>[4x]HPNYKLTYFNMRGRAEIIRYIFAYLDIQYEDHRIEQA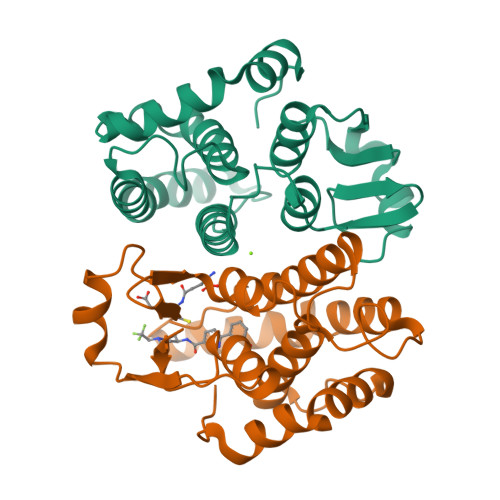DWPEIKSTLPFGKIPILEVDGLTLHQSLAIARYLTENTDLAGNTEMEQCHVDAIVDTLDDFMSCFPWAEKKQDVKEQMFNELLTYNAPHLMQDLDTYLGGREWLIGNSVTWADFYWEICSTTLLVFKPDLLDNHPRLVTLRKKVQAIPAVANWIKRRPQTKL> RVRSITLGNSTITTQECANVVVGYGVWPTYLNDDEATAEDQPTQPDVATCRFYTLESVMWQQSSPGWWWKFPDALSNMGLFGQNMQYHYLGRAGYTVHVQCNASKFHQGCLLVVCVP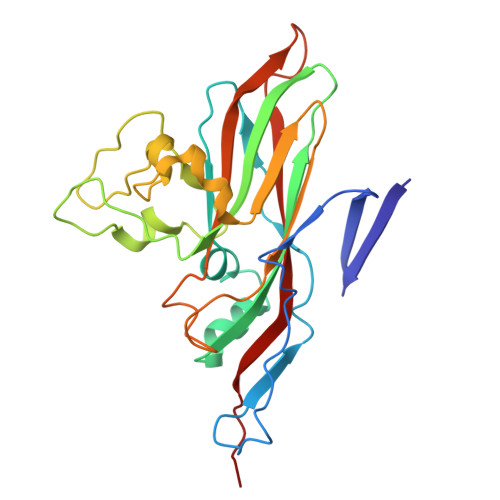EAEMGCATLANKPDQKSLSNGETANMFESQNSTGQTAVQANVINAGMGVGVGNLTIFPHQWINLRTNNSATIVMPYINSVPMDNMFRHNNFTLMIIPFAPLSYSTGATTYVPITVTVAPMCAEYNGLRLAG> SMAAFKPNSINYILGLDIGIASVGWAMVEIDEEENPIRLIDLGVRVFERAEVPKTGDSLAMARRLARSVRRLTRRRAHRLLRTRRLLKREGVLQAANFDENGLIKSLPNTPWQLRAAALDRKLTPLEWSAVLLHLIKHRGYLSQRKNEGETADKELGALLKGVAGNAHALQTGDFRTPAELALNKFEKESGHIRNQRSDYSHTFSRKDLQAELILLFEKQKEFGNPHVSGGLKEGIETLLMTQRPALSGDAVQKMLGHCTFEPAEPKAAKNTYTAERFIWLTKLNNLRILEQGSERPLTDTERATLMDEPYRKSKLTYAQARKLLGLEDTAFFKGLRYGKDNAEASTLMEMKAYHAISRALEKEGLKDKKSPLNLSPELQDEIGTAFSLFKTDEDITGRLKDRIQPEILEALLKHISFDKFVQISLKALRRIVPLMEQGKRYDEACAEIYGDHYGKKNTEEKIYLPPIPADEIRNPVVLRALSQARKVINGVVRRYGSPARIHIETAREVGKSFKDRKEIEKRQEENRKDREKAAAKFREYFPNFVGEPKSKDILKLRLYEQQHGKCLYSGKEINLGRLNEKGYVEIDAALPFSRTWDDSFNNKVLVLGSENQNKGNQTPYEYFNGKDNSREWQEFKARVETSRFPRSKKQRILLQKFDEDGFKERNLNDTRYVNRFLCQFVADRMRLTGKGKKRVFASNGQITNLLRGFWGLRKVRAENDRHHALDAVVVACSTVAMQQKITRFVRYKEMNAFDGKTIDKETGEVLHQKTHFPQPWEFFAQEVMIRVFGKPDGKPEFEEADTLEKLRTLLAEKLSSRPEAVHEYVTPLFVSRAPNRKMSGQGHMETVKSAKRLDEGVSVLRVPLTQLKLKDLEKMVNREREPKLYEALKARLEAHKDDPAKAFAEPFYKYDKAGNRTQQVKAVRVEQVQKTGVWVRNHNGIADNATMVRVDVFEKGDKYYLVPIYSWQVAKGILPDRAVVQGKDEEDWQLIDDSFNFKFSLH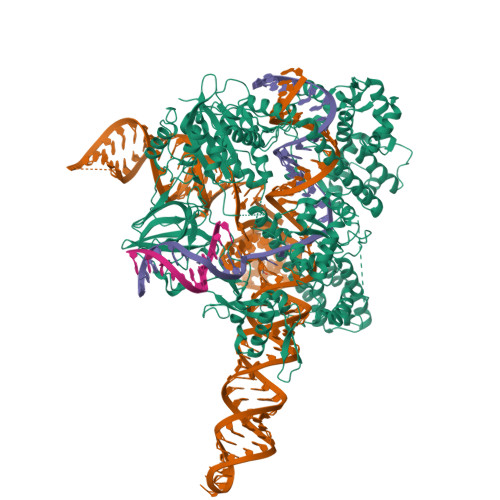PNDLVEVITKKARMFGYFASCHRGTGNINIRIHDLDHKIGKNGILEGIGVKTALSFQKYQIDELGKEIRPCRLKKRPPVR(4S,7R)-7-(heptanoyloxy)-4-hydroxy-N,N,N-trimethyl-10-oxo-3,5,9-trioxa-4-phosphahexadecan-1-aminium 4-oxide | C22 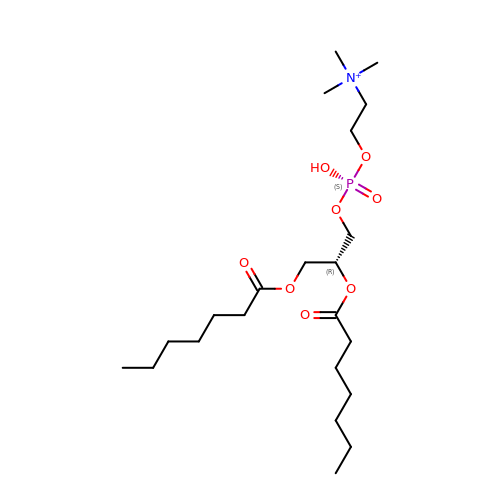H45 N O8 P | RBFSPQDASPEAID-HXUWFJFHSA-O> MGHMNITDIREQFPILHQQVNGHDLVYLDSAATSQKPRAVIETLDKYYNQYNSNVHRGVHTLGTRATDGYEGAREKVRKFINAKSMAEIIFTKGTTTSLNMVALSYARANLKPGDEVVITYMEHHANIIPWQQAVKATGATLKYIPLQEDGTISLEDVRETVTSNTKIVAVSHVSNVLGTVNPIKEMAKIAHDNGAVIVVDGAQSTPHMKIDVQDLDCDFFALSSHKMCGPTGVGVLYGKKALLENMEPAEFGGEMIDFVGLYESTWKELPWKFEAGTPIIAGAIGLGAAIDFLEEIGLDEISRHEHKLAAYALERFRQLDGVTVYGPEERAGLVTFNLDDVHPHDVATVLDAEGIAVRAGHHCAQPLMKWLDVTATARASFYLYNTEEEIDKLVEALQKTK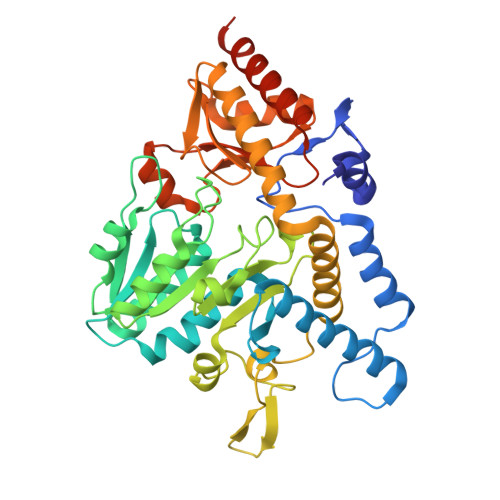EYFTNVFVDLEHHHHHH> SMRGALQLWQFLVALLDDPTNAHFIAWTGRGMEFKLIEPEEVARLWGIQKNRPAMNYDKLSRSLRYYYEKGIMQKVAGERYVYKFVCEPEALFSLAFPDNQRPALKAEFDRPVSEEDTVPLSHLDESPAYLPELA

The Ets transcription factor family consists of 28 genes in humans containing the evolutionarily conserved 85 amino acid Ets DNA-binding domain, originally identified as a viral oncogene (E26 transformation-specific). The Ets domain is a variant helix-turn-helix (winged helix) structure, comprising three α-helices and a four-stranded antiparallel β-sheet. Here, we present the crystal structures of the Ets domains of the entire PEA3 subfamily (Etv1, Etv4, and Etv5) together with the structure of the Erg family member (Fev). Furthermore, a new Ets dimerization interface linked by a redox-sensitive disulfide bond is identified, and this dimerization is shown to result in a significant inhibition of DNA binding, potentially linking Ets transcription factors with cellular redox regulatory mechanisms.

Crystals were obtained from constructs that contained the Ets domain, Etv1 (encompassing amino acids 326–429), Etv4 (encompassing amino acids 338–470), and Fev (encompassing amino acids 42–141). Etv1, Etv4, and Fev display the typical fold of the Ets domain, which contains three α-helices (α1–3) flanking a four-stranded β-sheet, with an additional C-terminal helix (α4). A comparison of the structures of Etv1, Etv4, and Fev in the presence and absence of DNA allows us to identify conformational changes that may occur upon DNA binding. In Etv4, in addition to three residues Arg-397, Arg-400, and Tyr-401 adopting different rotamers, the C-terminal end of the recognition helix switches from a 310 hydrogen bonding pattern (which is the form adopted in all the other ETS structures) to a more canonical α-helical hydrogen bonding pattern, although in this case the difference may be due to the fact an ethylene glycol molecule is bound in the vicinity. Analysis of the contacts between adjacent molecules in the Etv1, Etv4, and Etv5 crystals reveals a conserved potential dimer interface that is distant from the DNA binding surface and is present in all the DNA-free and DNA-bound crystal forms. This interface is centered around contributions from the N- and C-terminal helices, α1 and α4, with additional contacts involving residues from the β1-β2 loop. Dimerization of Etv1, -4, and -5 is mediated by the homologous cysteine residues (Cys-416, Cys-422, and Cys-449, respectively). Similarly, dimeric Etv4 and Etv5 also bind DNA with affinities that are 2 orders of magnitude lower than the reduced monomeric forms (note that the Kd values of the dimeric forms are rough estimates, as saturation could not be reached).naphthalene-1,3,6,8-tetrol | C10 H8 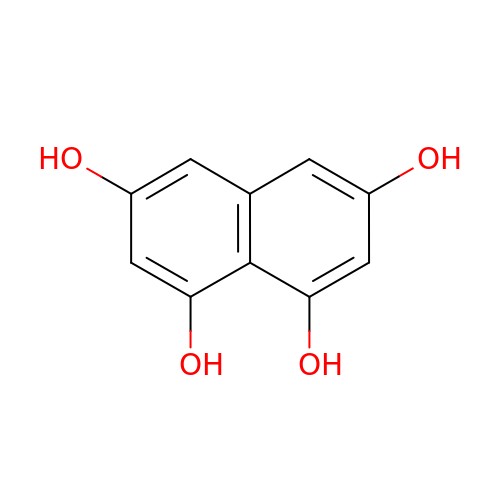O4 | BCMKHWMDTMUUSI-UHFFFAOYSA-N>METIQELILSEENKTNIAVLNLGTNDRRNAVLILETALHLVEKYLGKIINTSYLYETVPEYIVLDKKESCEKINKDCRIYDVNYINELMQNLEESKYEENKELIDKCEEYETFLKNGKVDNSILKEVNVENYLLECNNIIVKNDEIMKNNLSKYKDKYYTSYFYNLTVVVKTFVNDPLSMLVVIKYIEELMKRENVKEKEKFENRIIDIDILFFNDFTIFMKNIKLEKNMIYKILSKYIHLERDIKNGNDNMSKVNMDKDINLNNNNNIKKKNNNDIDCDCVDQKMNNHVNNKNYINSFRDPQEIINNMVDNIEFLSIPHVYTTHRYSILLCLNDMIPEYKHNVLNNTIRCLYNKYVSRMKEQYNINIKENNKRIYVLKDRISYLKEKTNIVGILNVNYDSFSDGGIFVEPKRAVQRMFEMINEGASVIDIGGESFGPFVIPNPKISERDLVVPVLQLFQKEWNDIKNKIVKCDAKPIISIDTINYNVFKECVDNDLVDILNDISACTNNPEIIKLLKKKNKFYSVVLMHKRGNPHTMDKLTNYDNLVYDIKNYLEQRLNFLVLNGIPRYRILFDIGLGFAKKHDQSIKLLQNIHVYDEYPLFIGYSRKRFITHCMNDQNVVINTQQKLHDEQQNENKNIVDKSHNWMFQMNYMRKDKDQLLYQKNICGGLAIASYSYYKKVDLIRVHDVLETKSVLDVLTKIDQVKD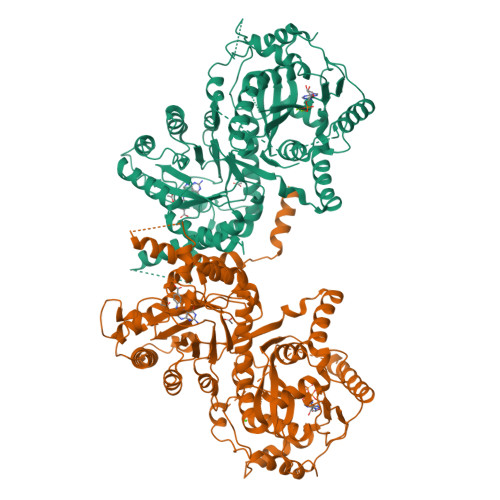PNSSSVDKLAAALEHHHHHH[2x]>APDTSVSNKQNFSTDVIYQIFTDRFSDGNPANNPTGAAFDGSCTNLRLYCGGDWQGIINKINDGYLTGMGITAIWISQPVENIYSVINYSGVNNTAYHGYWARDFKKTNPAYGTMQDFKNLIDTAHAHNIKVIIDFAPNHTSPASSDDPSFAENGRLYDNGNLLGGYTNDTQNLFHHYGGTDFSTIENGIYKNLYDLADLNHNNSSVDVYLKDAIKMWLDLGVDGIRVDAVKNMPFGWQKSFMATINNYKPVFTFGEWFLGVNEISPEYHQFANESGMSLLDFRFAQKARQVFRDNTDNMYGLKAMLEGSEVDYAQVNDQVTFIDNHDMERFHTSNGDRRKLEQALAFTLTSRGVPAIYYGSEQYMSGGNDPDNRARLPSFSTTTTAYQVIQKLAPLRKSNPAIAYGSTHERWINNDVIIYERKFGNNVAVVAINRNMNTPASITGLVTSLPRGSYNDVLGGILNGNTLTVGAGGAASNFTLAPGGTAVWQY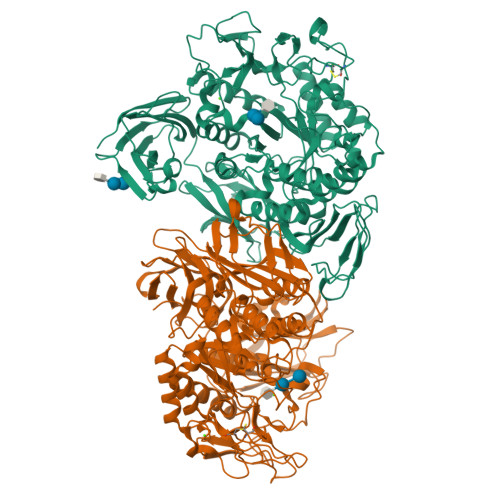TTDATTPIIGNVGPMMAKPGVTITIDGRGFGSGKGTVYFGTTAVTGADIVAWEDTQIQVKIPAVPGGIYDIRVANAAGAASNIYDNFEVLTGDQVTVRFVINNATTALGQNVFLTGNVSELGNWDPNNAIGPMYNQVVYQYPTWYYDVSVPAGQTIEFKFLKKQGSTVTWEGGANRTFTTPTSGTATVNVNWQP[2x]>MILVFLGPPGAGKGTQAKRLAKEKGFVHISTGDILREAVQKGTPLGKKAKEYMERGELVPD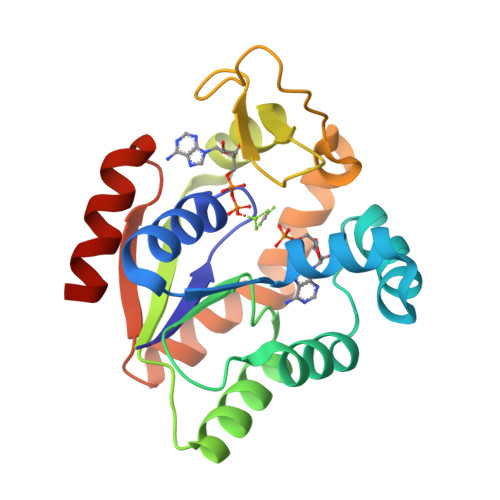DLIIALIEEVFPKHGNVIFDGFPRTVKQAEALDEMLEKKGLKVDHVLLFEVPDEVVIERLSGRRINPETGEVYHVKYNPPPPGVKVIQREDDKPEVIKKRLEVYREQTAPLIEYYKKKGILRIIDASKPVEEVYRQVLEVIGDGN[2x]>GAMPHDPSFTPTQLAARAAYLLRGNDLGTMTTAAPLLYPHMWSWDAAFVAIGLAPLSVERAVVELDTLLSAQWRNGMIPHIVFANGVDGYFPGPARWATATLADNAPRNRLTSGITQPPVHAIAVQRILEHARTRGRSTRAVAEAFLDRRWGDLMRWHRWLAECRDRNERGRITLYHGWESGMDNSPRWDSAYANVVPGKLPEYQRADNVIITDPSQRPSDGEYDRYLWLLEEMKAVRYDDERLPSVMSFQVEDVFFSAIFSVACQVLAEIGEDYKRPHADVKDLYLW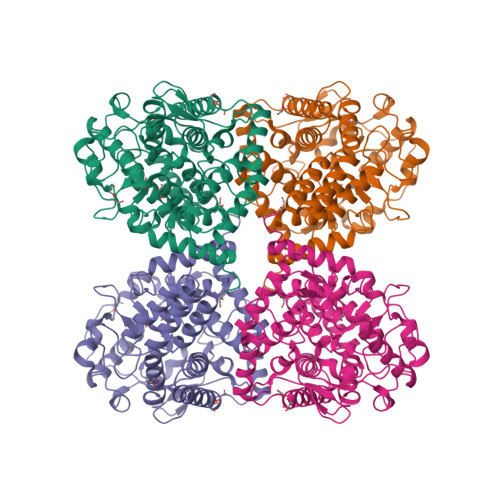AERFRAGVVETTDQRTGAARDFDVLAEKWLVTETAAQFAPLLCGGLPHDRERALLKLLEGPRFCGHPDLKYGLIPSTSPVSRDFRPREYWRGPVWPVLTWLFSWCFARRGWAERARLLRQEGLRQASDGSFAAYYEPFTGEPLGSMQQSWTAAAVLDWLG[2x]>MDPPVTHDLRVSLEEIYSGCTKKMKISHKRLNPDGKSIRNEDKILTIEVKKGWKEGTKITFPKEG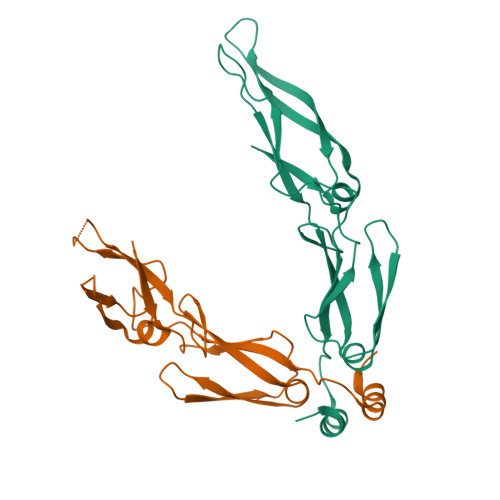DQTSNNIPADIVFVLKDKPHNIFKRDGSDVIYPARISLREALCGCTVNVPTLDGRTIPVVFKDVIRPGMRRKVPGEGLPLPKTPEKRGDLIIEFEVIFPERIPQTSRTVLEQVLPI[2x]>YPVKTDLHCRSSPSTSASIVRTYSSGTEVQIQCQTTGTSVQGSNVWDKTQHGCYVADYYVKTGHSGIFTTKCGSSSGGGSCKPPPINAATVALIKEFEGFVPKPAPDPIGLPTVGYGHLCKTKGCKEVPYSFPLTQETATKLLQSDIKTFTSCVSNYVKDSVKLNDNQYGALASWAFNVGCGNVQTSSLIKRLNAGENPNTVAAQELPKWKYAGGKVMPGLVRRRNAEVALFKKPSSVQAHPPKC[2x]

Muramidases are N-acetylmuramide glycanhydrolases which cleave the β-1,4-glycosidic bond between N-acetylmuramic acid (NAM) and N-acetylglucosamine (NAG) in the carbohydrate backbone of the bacterial cell-wall peptidoglycan. Here, the identification, characterization and X-ray structure of a novel fungal GH24 muramidase from Trichophaea saccata is first described, in which an SH3-like cell-wall-binding domain (CWBD) was identified by structure comparison in addition to its catalytic domain. A ‘domain-walking’ approach, searching for other sequences with a domain of unknown function appended to the CWBD, was then used to identify a group of fungal muramidases that also contain homologous SH3-like cell-wall-binding modules, the catalytic domains of which define a new GH family. The properties of some representative members of this family are described as well as X-ray structures of the independent catalytic and SH3-like domains of the Kionochaeta sp., Thermothielavioides terrestris and Penicillium virgatum enzymes.

Here, we report the identification of several new fungal GH24s with this CWBD and the structure of the intact T. saccata enzyme, henceforth referred to as TsCWBD-GH24. The linker, G73-SSSGGG-S80, appears to be flexible: its electron density is ill defined and it was not initially obvious how to assign the domains which compose a monomer. This was resolved by inspection of the surface, which strongly suggested a likely choice of connectivity for the domain pairs. While it is possible that the relative positions of the two domains is flexible in solution and that this particular orientation is a result of the crystal packing, we note that the linker is relatively short in this enzyme. The overall fold of the T. saccata catalytic GH24 domain follows that of the homologous GH24 enzymes. There is a clear decrease in activity when the CWBD is removed.> MSKIESALQAAQPGLSRLRGGAGGMGYRAATTQAEQPRSSLLDTIGRF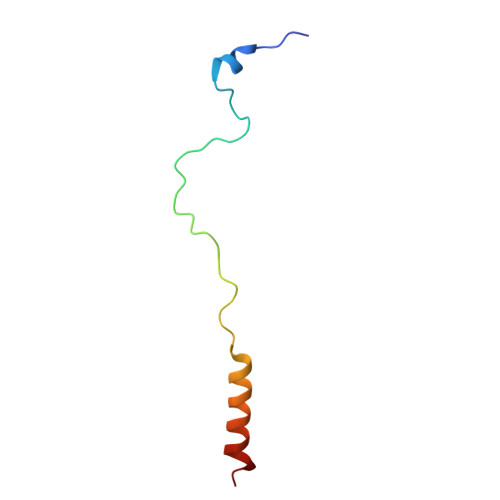AKAGADM> IIGGRESRPHSRPYMAYLQIQSPAGQSRCGGFLVREDFVLTAAHCWGSNINVTLGAHNIQRRENTQQHITARRAIRHPQYNQRTIQNDIML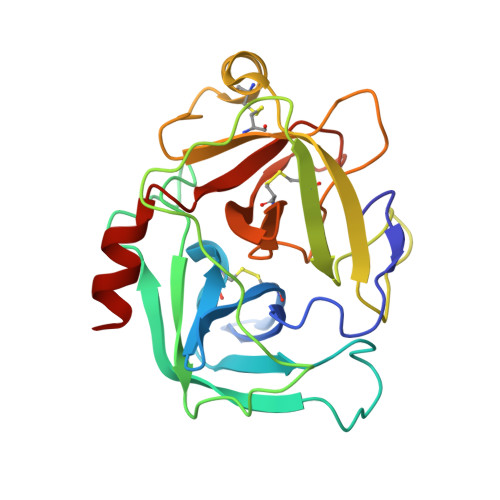LQLSRRVRRNRNVNPVALPRAQEGLRPGTLCTVAGWGRVSMRRGTDTLREVQLRVQRDRQCLRIFGSYDPRRQICVGDRRERKAAFKGDSGGPLLCNNVAHGIVSYGKSSGVPPEVFTRVSSFLPWIRTTMRS>ADTIVAVELNSYPNTDIGDPNYPHIGIDIKSIRSKSTARWNMQTGKVGTVHISYNSVAKRLSAVVSYSGSSSTTVSYDVDLNNVLPEWVRVGLSATTGLYKETNTILSWSFTSKLKTNSIADANSLHFSFHQFSQNPKDLILQGDAFTDSDG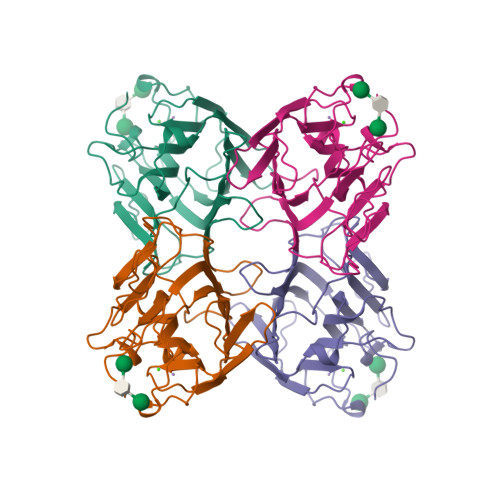NLELTKVSSSGDPQGNSVGRALFYAPVHIWEKSAVVASFDATFTFLIKSPDREPADGITFFIANTDTSIPSGSGGRLLGLFPDAN[2x]Transcription-repair coupling factors (TRCFs) are large superfamily 2 ATPases that mediate the preferential repair of the transcribed DNA strand (aka transcription-coupled DNA repair, TCR) in organisms ranging from bacteria to humans. At its core, TCR appears universally conserved, and relies on (1) the ability of transcription-repair coupling ATPases to release damage-stalled RNA polymerases (RNAPs) off the nucleic-acid template owing to ATP-driven translocation on dsDNA upstream of the transcription bubble, and (2) on their ability to recruit nucleotide excision repair (NER) machinery. In bacteria, a single protein, Mfd (aka TRCF) is necessary and sufficient for the coupling process. Mfd translocation on dsDNA is central to all Mfd functions.

Our observation that ADP•AlFx enhances the affinity for DNA allowed us to reconstitute stable Mfd-DNA complexes, and prepare specimens suitable for single-particle cryo-EM for structure determination. For our DNA substrate, we chose a 21mer blunt dsDNA fragment, consistent with previously determined Mfd footprints of ~26bp16,26,29. We thus acquired images at 30° tilts, which allowed us to obtain a more isotropic map resolved to 5.5 Å. This enabled us to readily dock all the individual domains of Mfd31 into the map and perform real-space refinement to obtain the final model. At this resolution, we do not observe density that can be assigned to the transition state analog moiety. First, our reconstruction reveals an unexpected large-scale swiveling motion of the UvrB homology module (D1a-D2-D1b), which results in a ~49 Å displacement and an 82° rotation of D2. Second, particularly striking is the repositioning of domain of unknown function D3, which swings from the ventral side laterally toward D7 upon DNA binding, establishing new bridging interactions with the UvrB homology module and D7. In contrast, when Mfd is bound to DNA, D3 makes contacts with D1a and D7, swapping position with D2. The UvrA-binding surface on D2, including residues critical for binding such as R165 and R18129 becomes fully exposed. In our reconstruction, the two helices of the TRG snap together and are likely stabilized by ADP•AlFx. binding.

> HHHHHHSSGLEVLFQGPHMASMPEQYRYTLPVKAGEQRLLGELTGAACATLVAEIAERHAGPVVLIAPDMQNALRLHDEISQFTDQMVMNLADWETLPYDSFSPHQDIISSRLSTLYQLPTMQRGVLIVPVNTLMQRVCPHSFLHGHALVMKKGQRLSRDALRTQLDSAGYRHVDQVMEHGEYATRGALLDLFPMGSELPYRLDFFDDEIDSLRVFDVDSQRTLEEVEAINLLPAHEFPTDKAAIELFRSQWRDTFEVKRDPEHIYQQVSKGTLPAGIEYWQPLFFSEPLPPLFSYFPANTLLVNTGDLETSAERFQADTLARFENRGVDPMRPLLPPQSLWLRVDELFSELKNWPRVQLKTEHLPTKAANANLGFQKLPDLAVQAQQKAPLDALRKFLETFDGPVVFSVESEGRREALGELLARIKIAPQRIMRLDEASDRGRYLMIGAAEHGFVDTVRNLALICESDLLGERVARRRQDSRRTINPDTLIRNLAELHIGQPVVHLEHGVGRYAGMTTLEAGGITGEYLMLTYANDAKLYVPVSSLHLISRYAGGAEENAPLHKLGGDAWSRARQKAAEKVRDVAAELLDIYAQRAAKEGFAFKHDREQYQLFCDSFPFETTPDQAQAINAVLSDMCQPLAMDRLVCGDVGFGKTEVAMRAAFLAVDNHKQVAVLVPTTLLAQQHYDNFRDRFANWPVRIEMISRFRSAKEQTQILAEVAEGKIDILIGTHKLLQSDVKFKDLGLLIVDEEHRFGVRHKERIKAMRANVDILTLTATPIPRTLNMAMSGMRDLSIIATPPARRLAVKTFVREYDSMVVREAILREILRGGQVYYLYNDVENIQKAAERLAELVPEARIAIGHGQMRERELERVMNDFHHQRFNVLVCTTIIETGIDIPTANTIIIERADHFGLAQLHQLRGRVGRSHHQAYAWLLTPHPKAMTTDAQKRLEAIASLEDLGAGFALATHDLEIRGAGELLGEEQSGSMETIGFSLYMELLENAVDALKAGREPSLEDLTSQQTEVELRMPSLLPDDFIPDVNTRLSFYKRIASAKTENELEEIKVELIDRFGLLPDPARTLLDIARLRQQAQKLGIRKLEGNEKGGVIEFAEKNHVNPAWLIGLLQKQPQHYRLDGPTRLKFIQDLSERKTRIEWVRQFMRELEENAIA> MSVIVYRNNQSTLTLNGYTFQHLYQGAALVLTPVNAKTARTNSINGGVSISGRVDGGVHTLAIMVQKHSPDDKFLNDAKNSQEPVVFDGSMK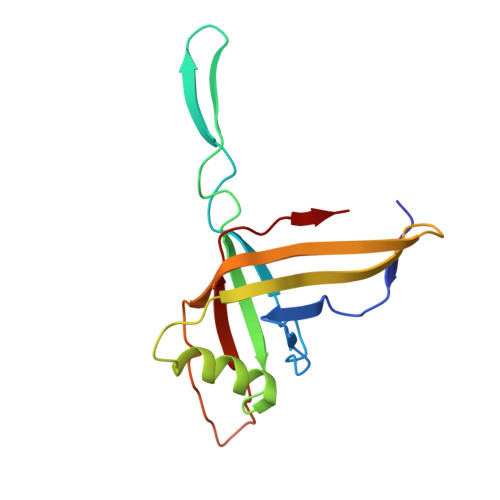RAYTESGTLKKATTTLETGSITTQPTKTDNNQDPDDSRTYVIEFRNSVETF> DSISTRGLFGAIAGFLEGGWDGMIAGWHGYSSTGDHGTKVAADLVSTQKAMDAITARINNMNKMTERAFSVTDSTMQEIQKEIKDLDKKIDDVRADETAAQIEMIVLLENENI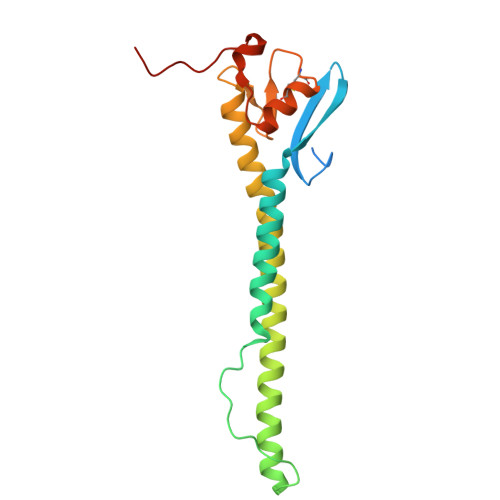INAEDEHVHALKQKLTKMLGPSAQDMGDGCFIVDHQCKEDCLREIVSGNYTPSKYGMDEFKSPIITGT> QVDVHDPVMTREGDTWYLFSTGPGITIYSSKDRVNWRYSDRAFATEPTWAKRVSPSFDGHLWAPDIYQHKGLFYLYYSVSAFGKNTSAIGVTVNKTLNPASPDYRWEDKGIVIESVPQRDLWNAIDPAIIADDHGQVWMSFGSFWGGLKLFKLNDDLTRPAEPQEWHSIAKLERSVLMDDSQAGSAQIEAPFILRKGDYYYLFASWGLCCRKGDSTYHLVVGRSKQVTGPYLDKTGRDMNQGGGSLLIKGNKRWVGLGHNSAYTWDGKD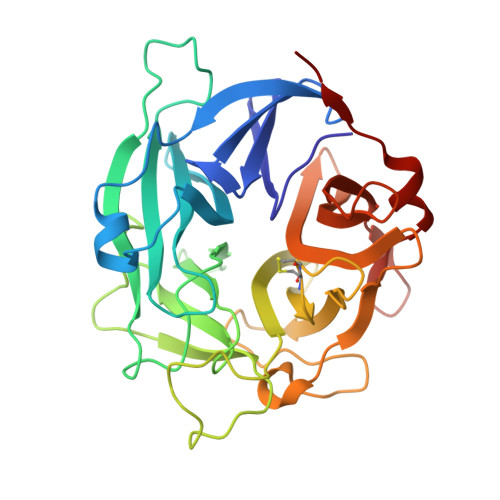YLVLHAYEAADNYLQKLKILNLHWDGEGWPQVDEKELDSYISQRLK> XELEAIAQKFEAIAKKFEA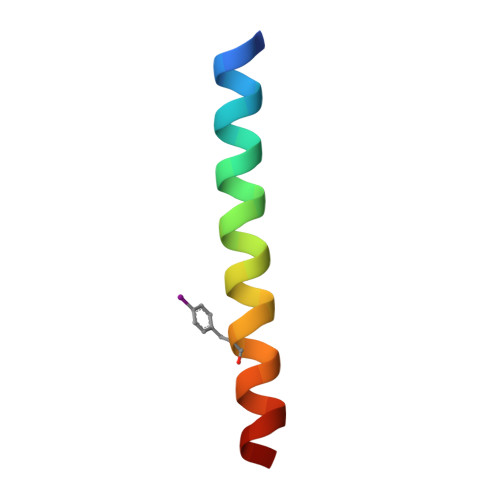IAFKFEAIAQKX> DRHHHHHHKLSPANDDQSRPSLSNGHTCVGCVLVVSVIEQLAQVHNSTVQASMERLCSYLPEKLFLKTTCYLVIDKFGSDIIKLLSADMNA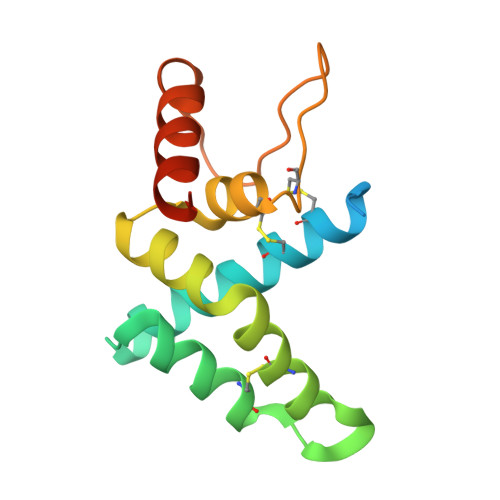DVVCHTLEFCKQNTGQPLCHLYPLPKETWKFTLQKARQIVKKSPILKY> TTPLVHVASVEKGRSYEDFQKVYNAIALKLREDDEYDNYIGYGPVLVRLAWHTS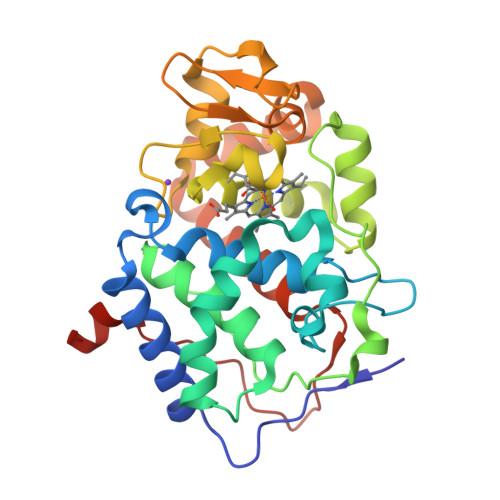GTWDKHDNTGGSYGGTYRFKKEFNDPSNAGLQNGFKFLEPIHKEFPWISSGDLFSLGGVTAVQEMQGPKIPWRCGRVDTPEDTTPDNGRLPDADKDADYVRTFFQRLNMNDREVVALSGAHTLGKTHLKNSGYEGPWTANNNVFDNSFYLNLLNEDWKLEKNDANNEQWDSKSGYLQLPTDYSLIQDPKYLSIVKEYANDQDKFFKDFSKAFEKLLENGITFPKDAPSPFIFKTLEEQGL(7S)-2-[(3,5-difluoro-4-hydroxyphenyl)amino]-5,7-dimethyl-8-(3-methylbutyl)-7,8-dihydropteridin-6(5H)-one 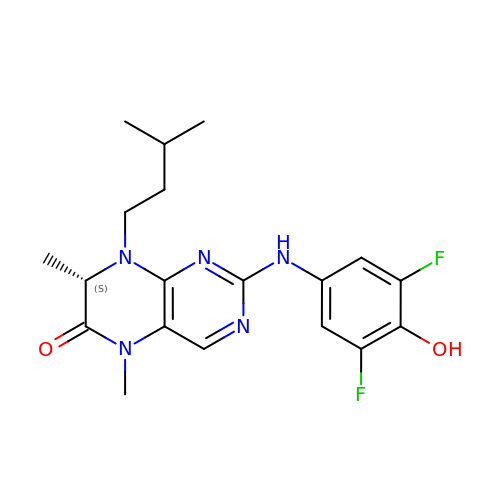| C19 H23 F2 N5 O2 | DTEKTGDVSARYDS-NSHDSACASA-N>SNASTVATYSYTHSVTYVTDNILKSLKDIILLSGLDPEHFADRWESNTRAIKTWLGTGDLRKVILEIYNPATDKLVTRWDIDIVYGWSDGDGSFWTDTEQLKYAIKKAGLLPSQAKY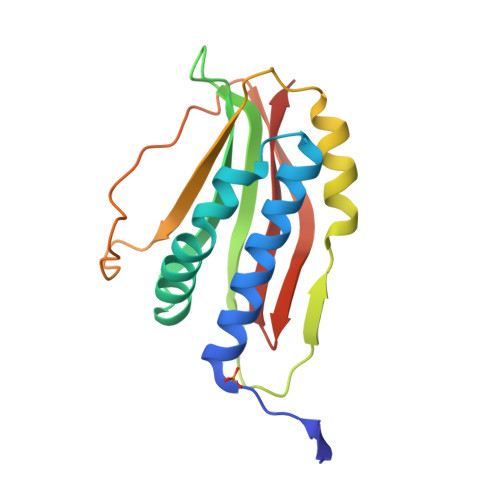KLMLDTKPGRPDVEGWSKGSYRSTDGMVKQSLGSTVEHSGLAGQAGYWRQR[4x]1-tert-butyl-3-[(3-chlorophenyl)methyl]-1H-pyrazolo[3,4-d]pyrimidin-4-amine | C16 H18 Cl N5 | 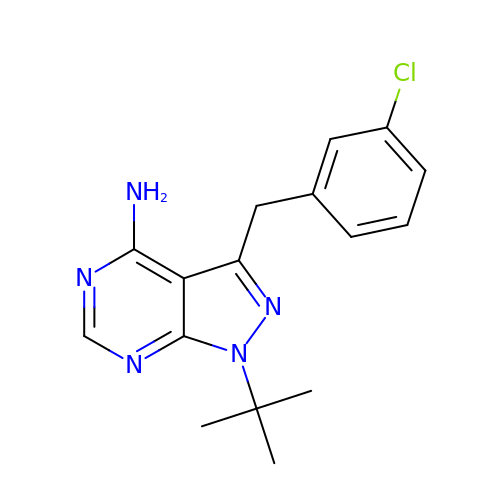VYDBKDXQXXHCLQ-UHFFFAOYSA-N>[2x]GSMTEIALIGNPNSGKTSLFNLITGHNQRVGNWPGVT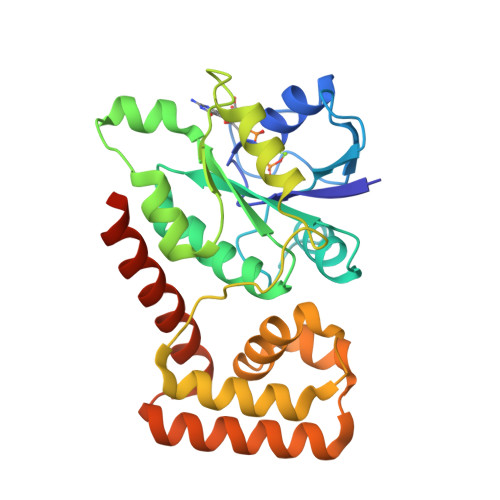VERKSGLVKKNKDLEIQDLPGIYSMSPYSPAEKVARDYLLSQRADSILNVVDATNLERNLYLTTQLIETGIPVTIALNMIDVLDGQGKKINVDKLSYHLGVPVVATSALKQTGVDQVVKKAAHTTTSTVGDLAFPIYDDRLEAAISQILEVLGNSVPQRSARFYAIKLFEQDSLVEAELDLSQFQRKEIEDIIRITEEIFTEDAESIVINERYAFIERVCQMAESHTEDFALTLS> GHSSSDPVYPCGICTNEVNDDQDAILCEASCQKWFHRICTGMTETAYGLLTAEASAVWGCDTCMA;> AMAAKVVYVFSTEMANKAAEAVLKGQVETIVSFHI

Pygo and BCL9/Legless transduce the Wnt signal by promoting the transcriptional activity of β-catenin/Armadillo in normal and malignant cells. Molecularly, BCL9/Lgs proteins function as adaptors between Pygo and Armadillo/β-catenin, by binding through their homology domain 1 (HD1) to the PHD finger in the C terminus of Pygo, and through their homology domain 2 (HD2) to the Armadillo repeat domain of Armadillo/β-catenin (Kramps et al., 2002; Städeli and Basler, 2005). We show that human and Drosophila Pygo PHD fingers associate with their cognate HD1 domains from BCL9/Legless to bind specifically to the histone H3 tail methylated at lysine 4 (H3K4me). Therefore, this is a prime example of histone tail binding by a PHD finger (of Pygo) being modulated by a cofactor (BCL9/Legless).

To understand how Pygo proteins interact with BCL9, we coexpressed the PHD finger from hPygo1 with its cognate HD1 domain from human BCL9 in bacteria, and purified the resulting complex (hPHD-HD1, the “binary complex”), which was stable over gel filtration and exhibited equimolar binding. It produced diffracting crystals in several different crystallization conditions, which enabled us to determine its structure by X-ray crystallography at 1.59 Å resolution. The binary complex shows a segregation of charges on its molecular surface, with one face being predominantly negatively, and the opposite positively, charged. The former presents two conspicuous hydrophobic cavities (arrows) surrounded by acidic residues and separated by W366, similar to the histone-binding pockets seen in other PHD fingers. Two sets of contacts mediate the interaction between hPHD and HD1. The first involves primarily β sheet H bonds between PHD β5 (S387, V389, and G391) and HD1 β1 (Y178, V179, and F180). These intermolecular interactions depend mainly on backbone atoms. The second set of contacts comprises a network of hydrophobic side chains, as well as two H bonds (formed by HD1 N186 side chains and PHD backbone atoms). These side-chain contacts involve either invariant residues (T375, A378, and L382) or a semiconserved PHD residue (M374). Likewise, the HD1 residues involved in these hydrophobic interactions are either invariant (T182, A185, N186, A189, and I200) or semiconserved (V201).> LSCRWVDHKF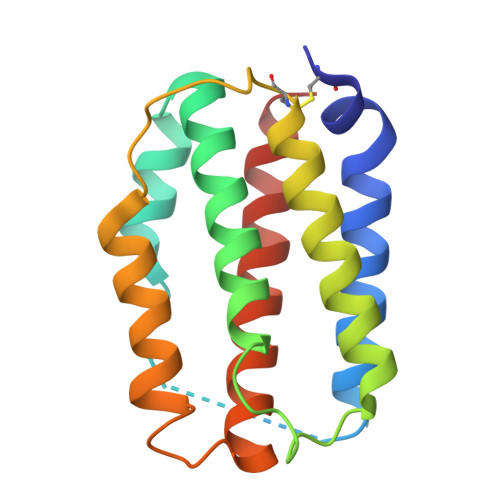RQHSETSLDLLNTMANNSTNSTEDAQVEDTVAFPNDLYSQASKASAEDKLHFTVQVLEEAAALFEEDHSNASWEENTVENFVNVVNQQADGLRSCTGSHGHKKKNKKLHMYFKRLSSHVLKKMSHSAEAWELIRKEIRTHLMRADQLVSSLRNTN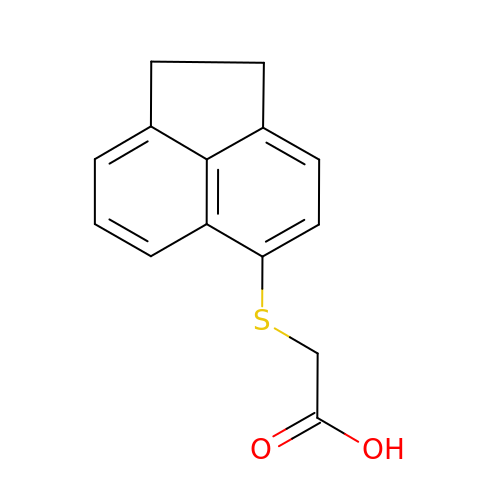2-(1,2-dihydroacenaphthylen-5-ylsulfanyl)ethanoic acid | C14 H12 O2 S | ILIYQPKGPUGGBV-UHFFFAOYSA-N>[16x]FTLIELLIVIAIIAILAAVLIPNLLAARKRANDTVVTAYLNDAVKFQEMYQIDNNSYTSNQAALISLGLKSTPANVTFSIVSASANSYCMIAGHSGGTVWFAATPDKGVYKTNTAVTSSQPESCP

Type IV pili (T4P) are flexible extracellular protein filaments found on many bacteria. They form multifunctional fibres involved in twitching motility, adhesion, immune evasion, bacteriophage infection, virulence and colony formation. Pilins have a conserved N-terminal α-helix, with a 4–5 stranded antiparallel β-sheet at the C-terminus. The α-helix forms the core of the filament, while the globular β-sheet head domain is solvent exposed and subject to post-translational modification.

Our data unambiguously demonstrate that the wider pilus is composed of the major pilin PilA4. The diameter of the wide pilus is 70 Å and is roughly cylindrical. The region between the N-terminal α-helix and the C-terminal β-sheet, the so-called glycosylation loop, ranges in PilA4 from amino acids 55–77, with a two-turn α-helix comprising amino acids 61–67. The C-terminal region is an antiparallel four-stranded β-sheet with the last strand facing towards the N-terminus followed by a loop that ends on the β-sheet. A disulphide bond between Cys89, which is located in the second strand, and the penultimate amino acid Cys124, likely stabilises the C-terminus. PilA4 has no net charge but the filament displays a distinctive positively charged groove along the filament axis. In the wide (PilA4) filament, each subunit (subunit A) interacts with the N-termini that project down from the next two subunits above (B and C) and from the subunits which are six and seven subunits above (G and H). PilA4 contains two intermolecular salt bridges—between Asp53 (subunit A) and Arg30 (subunit D), and between Glu48 (subunit A) and Arg28 (subunit E). The surface of our wide PilA4 filaments show a striking line of positively charged residues along the long axis, into which a double stranded DNA molecule can be fitted. In summary, we conclude that PilA4 has three known roles: it promotes pilus formation for both wide and narrow filaments, it comprises the main structure of the wide T4P, and it plays a role in natural transformation.The O-acetylation of alginate requires the concerted action of four proteins: the putative MBOAT protein, AlgI; a protein of unknown function, AlgF; and two annotated O-acetyltransferases AlgJ and AlgX. AlgI is predicted to be a member of the MBOAT family, while AlgJ and AlgX are required in the O-acetylation of alginate as the polymer passages through the periplasm. The TMHMM server v2.0 indicates that AlgJ from P. aeruginosa PAO1 possesses a transmembrane helix from residues 12–29 that tethers the periplasmic domain to the cytoplasmic membrane; a prediction that is supported by in vivo localization studies. AlgJ exhibits acetylesterase activity that is mediated through the Ser-His-Asp catalytic triad similar to that of the SGNH hydrolase-like enzyme AlgX.

To this end, we have determined the structure of Pseudomonas putida AlgJ75–370 (PpAlgJ75–370) to 1.83 Å resolution and have functionally characterized the protein. Selenomethionine-incorporated (SeMet) protein was expressed, purified, crystallized, and the structure determined to 1.83 Å using the single-wavelength anomalous dispersion (SAD) technique. PpAlgJ75–370 crystallized in space group C2 with two molecules in the asymmetric unit. The dimer observed in the crystal structure is therefore not believed to be biologically relevant. SGNH hydrolases have an α/β/α fold with each of the four conserved active site residues responsible for catalysis residing in one of four conserved blocks. The structure of PpAlgJ75–370 reveals that the protein has an α/β/α fold with a core of four parallel β-strands (Figure 1: β3, β6–8) and an isolated β-bridge at β3, which are comparable to the five parallel β-strands found in canonical SGNH hydrolases. A surface representation of PpAlgJ75–370 reveals a shallow groove that crosses the face of the protein (left, centre). In PpAlgJ the corresponding residues D190 and H192 are located in the shallow electronegative groove (centre). The active site of PpAlgJ75–370 and the orientation of the putative catalytic triad D190, H192 and S288, is analogous to PaAlgX27–474 and other serine esterases and proteases. Examination of the PpAlgJ75–370 structure suggests that Y348 is in a position to act as a hydrogen bond donor in place of the conserved asparagine. AlgJ appears to be a circularly permuted member of SGNH hydrolases as the order of conserved residues in primary sequence (H-S-G-Y) is different than that of SGNH hydrolases (S-G-N-H).

>[2x]GSHMNEGRPGVVLGRDQWLFSDEEFKPTAGAEQLMQENLALIRGVRDTLQQHGSQLVLAIVPAKARVYTEYLGKERPASLHDDLYNQFHAQARQANVFAPDLMAPMEQAKARGQVFLRTDTHWTPMGAEVAAQALAEAVSRQSLLNGDPQAFITEAGNTAPYKGDLTNFLPLDPLFSNLLPAPDNLQKRTTRPVDAEGDAGDALFADKQIPVALVGTSYSANPHWNFLGALQQALRSDVANYAEDGHGPLLPMLKYLQSDAFKNAAPQVVVWEFPERYLPMKNDLSSFDPQWIAQLKNSRLEHHHHHH> GDVEEAIERAVVHVADTMRSGPSNSASVPALTAVETGHTSQVTPSDTMQTRHVKNYHSRSESTVENFLGRSACVYMEEYKTTDNDVNKKFVAWPINTKQMVQMRRKLEMFTYLRFDMEVTFVITSRQDPGTTLAQDMPVLTHQIMYVPPGGPIPAKVDDYAWQTSTNPSIFWTEGNAPARMSIPFISIGNAYSNFYDGWSNFDQRGSYGYNTLNNLG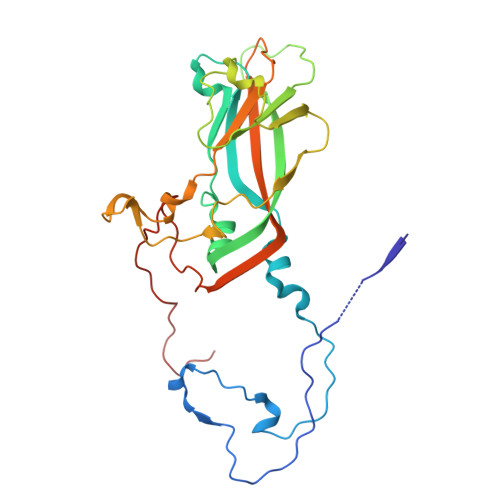HIYVRHVSGSSPHPITSTIRVYFKPKHTRAWVPRPPRLCQYKKAFSVDFTPTPITDTRKDINTVTT>MSTLIPPPSKKQKKEAQLPREVAIIPKDLPNVSIKFQALDTGDNVGGA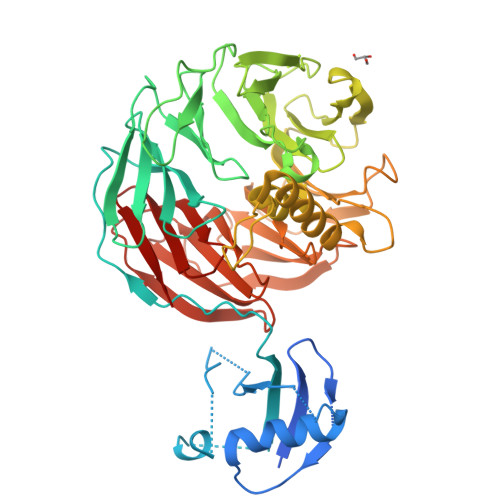LRVPGAISEKQLEELLNQLNGTSDDPVPYTFSCTIQGKKASDPVKTIDITDNLYSSLIKPGYNSTEDQITLLYTPRAVFKVKPVTRSSSAIAGHGSTILCSAFAPHTSSRMVTGAGDNTARIWDCDTQTPMHTLKGHYNWVLCVSWSPDGEVIATGSMDNTIRLWDPKSGQCLGDALRGHSKWITSLSWEPIHLVKPGSKPRLASSSKDGTIKIWDTVSRVCQYTMSGHTNSVSCVKWGGQGLLYSGSHDRTVRVWDINSQGRCINILKSHAHWVNHLSLSTDYALRIGAFDHTGKKPSTPEEAQKKALENYEKICKKNGNSEEMMVTASDDYTMFLWNPLKSTKPIARMTGHQKLVNHVAFSPDGRYIVSASFDNSIKLWDGRDGKFISTFRGHVASVYQVAWSSDCRLLVSCSKDTTLKVWDVRTRKLSVDLPGHKDEVYTVDWSVDGKRVCSGGKDKMVRLWTH[2x]>[2x]MIVTSGVLVENGKVLLVKHKRLGVYIYPGGHVEHNETPIEAVKREFEEETGIVVEPIGFTYGIIDENAVERPM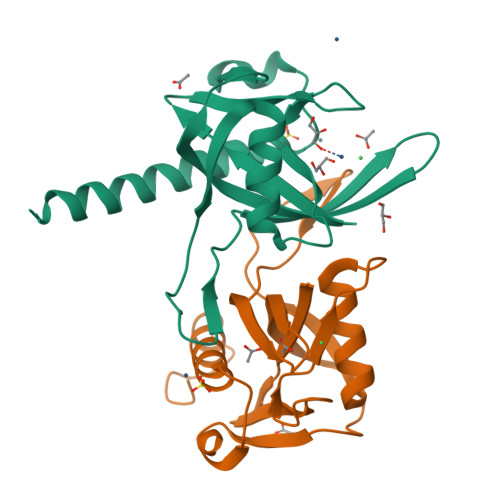PLVILEEVVKYPEETHIHFDLIYLVKRVGGDLKNGEWIDVREIDRIETFPNVRKVVSLALSTLYRLGKISKLAAALEHHHHHH>APLAQRVRIMGGTNRGRAEVYYNNEWGTICDDDWDNNDATVFCRMLGYSRGRALSSYGGGSGN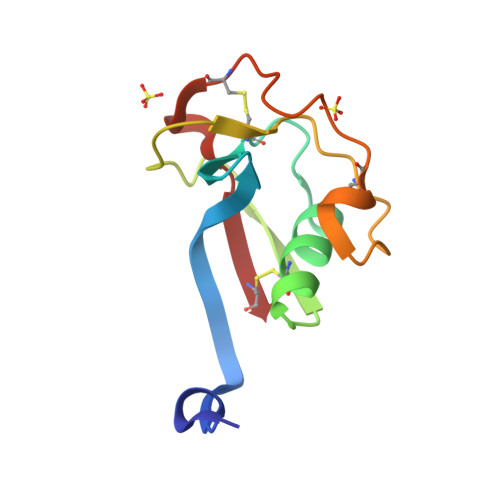IWLDNVNCRGTENSLWDCSKNSWGNHNCVHNEDAGVECS[2x]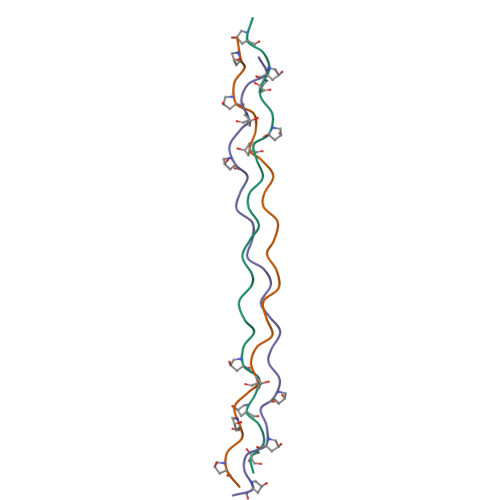>[3x]PPGPPGPPGFPGMKGHRGFDGPPGPPGPPG>MDIMNEKVKKIIEFMDKNSIDAVLIAKNPNVYYISGASPLAGGYILITGESATLYVPELEYEMAKEESNIPVEKFKKMDEFYKALEGIKSLGIESSLPYGFIEELKKKANIKEFKKVDDVIRDMRIIKSEKEIKIIEKACEIADKAVMAAIEEITEGKKEREVAAKVEYLMKMNGAEKPAFDTIIASGYRSALPHGVASDKRIERGDLVVIDLGALYQHYNSDITRTIVVGSPNEKQKEIYEIVLEAQKKAVESAKPGITAKELDSIARNIIAEYGYGEYFNHSLGHGVGLEVHEWPRVSQYDETV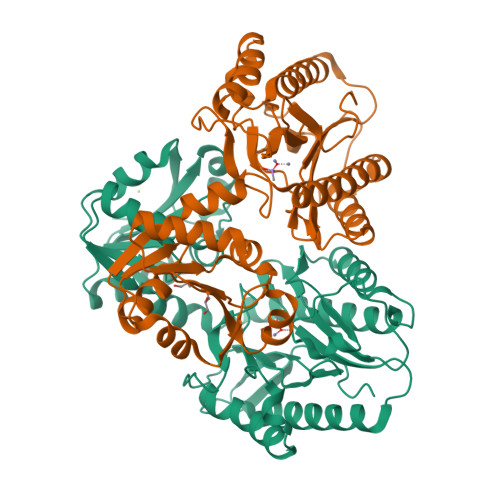LREGMVITIEPGIYIPKIGGVRIEDTILITKNGSKRLTKTERELI[2x]>[2x]FDKMQAHIGEVNGTISIGCSSLIGQTLLPEVLSLYNAQFPNVEIQVQVGSTEQIKANHRDYHVMITRGNKV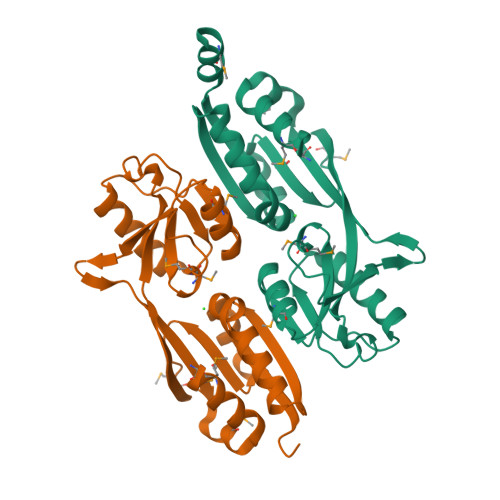MNLANTHLFNDDHYFIFPKNRRDDVTKLPFIEFQADPIYINQIKQWYNDNLEQDYHATITVDQVATCKEMLISGVGVTILPEIMMKNISKEQFEFEKVEIDNEPLIRSTFMSYDPSMLQLPQVDSFVNLMASF> MKESLKDRIRLWKRLYVNAFENALNAIPNVKGVLLAYNTNIDAIKYLDKDDLEKRVTEIGKEKVFEIIENPPEKISSIEELLGGILRSIKLGKAMEWFVESEEVRRYLREWGWDELRIGGQAGIMANLLGGVYRIPTIVHVPQNPKLQAELFVDGPIYVPVFEGNKLKLVHPKDAIAEEEELIHYIYEFPRGFQVFDVQAPRENRFIANADDYNARVYMRREFREGFEEITRNVELAIISGLQVLKEYYPDGTTYRDVLDRVESHLNILNRYNVKSHFEFAYTANRRVREALVELLPKFTSVGLNEVELASIMEIIGDEELAKEVLEGHIFSVIDAMNVLMDETGIERIHFHTYGYYLALTQYRGEEVRDALLFASLAAAAKAMKGNLERIEQIRDALSVPTNERAIVLEEELEKEFTEFENGLIDMVDRQLAFVPTKIVASPKSTVGIGDTISSSAFVSEFGMRKR

One of these major differences is the presence of ADP-dependent glucokinases (GKs) and phosphofructokinases (PFKs), instead of the classical ATP-dependent kinases. Even though these ADP-dependent kinases show no sequence similarity to ATP-dependent enzymes known to date, the determination of their three dimensional structures allowed their reliable classification as members of the ribokinase superfamily. In addition to this core ribokinase-like fold; other members of this superfamily have an extra small domain, which in the case of the ADP-dependent kinases is formed by a five stranded β-sheet with some α-helical insertions, the active site lying between the two domains. Our results indicated that Mg·AMP behaves as a competitive inhibitor of Mg·ADP and as a mixed type inhibitor with respect to D-glucose; the other product, D-glucose-6-P presents a mixed type inhibition versus either Mg·ADP or D-glucose. These patterns of inhibition are consistent with an ordered sequential mechanism in which Mg·ADP is the first substrate to bind to the catalytic site and Mg·AMP the last product to be released.

We determined the crystal structures of TlGK in its apo form (absence of ligands) and holo form, in the presence of D-glucose and the nonhydrolyzable ADP analog ADPβS (ternary complex, ADPβS·D-glucose). Both structures were obtained by molecular replacement, and refined to 2.05 and 2.58 Å resolution, respectively. The overall structure of TlGK in both states (apo-enzyme and ternary complex) shows the same two domains organization described previously; the large domain harbors a Rossmann fold (α/β/α) architecture with a central twelve stranded β-sheet surrounded by thirteen α-helices and three 310 helices, and the small inserted domain consisting of five β-strands and four α-helices. When the enzyme is in ligand-free state (apo), the large and small domains are distant from each other and accordingly there are no discernible interactions between residues from either domain. In the absence of ligands, the mass centers of the small and large domain were separated by 29.4 Å, but when Mg·ADPβS and D-glucose were simultaneously bound to the active site, the two domains underwent conformational changes causing the inter-domain distance to shrink by nearly 3 Å, that to 26.5 Å. Cluster 2 involves Arg202 (small domain) and Tyr354 (large domain). The distance between the two side-chain groups is reduced from 12.0 Å in the apo-enzyme to only 3.4 Å in the ternary complex (cluster 2). Cluster 5 is defined by interactions between residues Lys74 and Lys246 located in the small and large domain, respectively. In the apo-enzyme the distance between amine groups is >8.7 Å, whereas in the ternary complex this distance decrease to 4.0 Å, close enough to establish a repulsive interaction between the side chains of these Lys residues. For the apo-enzyme, the SAXS ab initio model suggests a more open conformation than the one found in the crystal.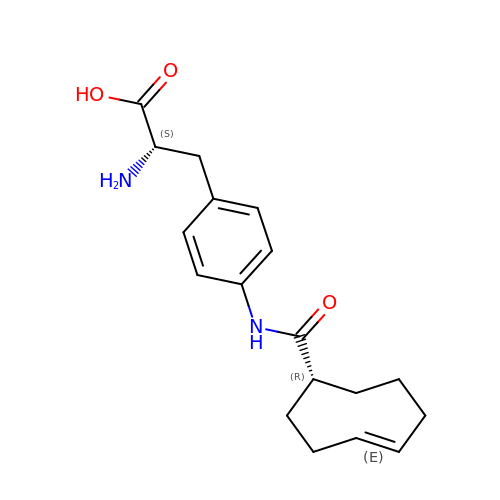4-{[(1R,4E)-cyclooct-4-en-1-ylcarbonyl]amino}-L-phenylalanine | C18 H24 N2 O3 | NTVNNTNXRKFWIK-BJEUKDNBSA-N> ASTLKSGSKEVENLKKPFMPPREVHVQVTHSMPPQKIEIFKSLDNWAEENILVHLKPVEKCWQPQDFLPDPASDGFDEQVRELRERAKEIPDDYFVVLVGDMITEEALPTYQTMLNTLDGVRDETGASPTSWAIWTRAWTAEENRHGDLLNKYLYLSGRVDMRQIEKTIQYLIG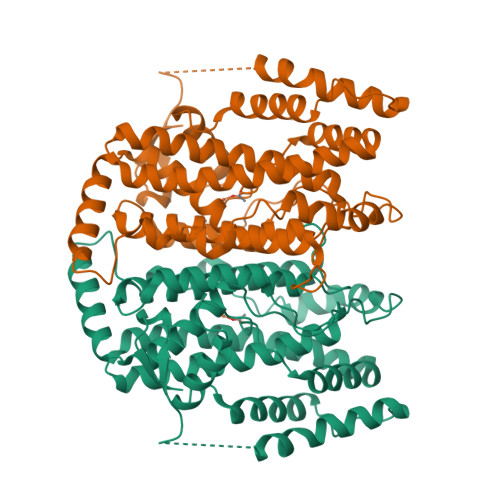SGMDPRTENSPYLGFIYTSFQERATFISHGNTARQAKEHGDIKLAQICGTIAADEKRHETAYTKIVEKLFEIDPDGTVLAFADMMRKKISMPAHLMYDGRDDNLFDHFSAVAQRLGVYTAKDYADILEFLVGRWKVDKLTGLSAEGQKAQDYVCRLPPRIRRLEERAQGRAKEAPTMPFSWIFDRQVKL>[2x]MAHHHHHHVDDDDKMVTAAKGRIIGYVPGWKTPPAAQELASAGYTHVMIAFGVFSTNTPGVIVPAFETITKEYIQSL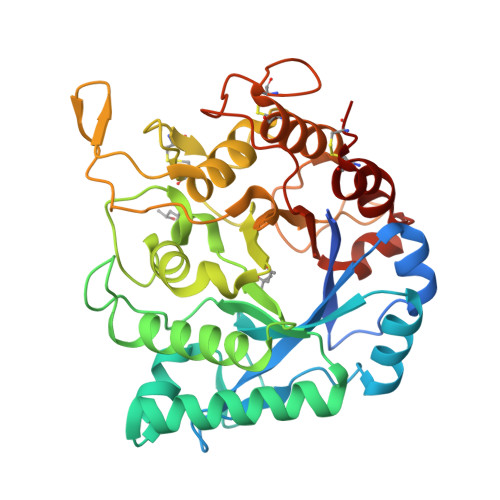HQAGIKVILSLGGALTSIPNTTVDFHQVLVASSSPEAFKQTFINSLKELISQYGFDGFDTDIEHGINASGSFSQPQGDIAVLASIINTMYSQNSSLLITLTPQVANIAATSGFDQTWGNYASLIMQTHQSLAWVGIQLYNTGCAFGIDQVCYGPTPTDTPDFSVAMATDLLENWPATVNGRPTGFQPYISYLRPSQIVIGYPSPNASGGSDGSPVTPTTTIKRAIQCLKTAIAGNTSCGVYVPPRAYGNIGGVFNWEVTYDKNNQFKFAKELKNCAINGVCE The Lon protease is a AAA+ protein found in prokaryotes, archaea, and eukaryotic organelles. Lon is involved in cellular protein homeostasis by degrading damaged or misfolded abnormal proteins, which prevents these unwanted protein species from forming toxic aggregates. Lon is known to form a homohexamer; each protomer is composed of multiple domains, including an N-terminal substrate-binding globular domain (NGD), a long-helix domain (LH), a three-helix bundle (3H), a AAA+ ATPase module, and a protease domain. We show here, using cryo-electron microscopy (cryo-EM), that the activation process of the Lon AAA+ protease may involve a pentameric assembly and a substrate-dependent incorporation of the sixth protomer to form the substrate-pore-loop contacts seen in the translocating state.

To create monomeric mutants, we designed ΔN-E613K and ΔN-L708R mutations, each of which would introduce a positive charge to the hydrophobic interface. If the ΔN-E613K and ΔN-L708R proteins are monomeric, they are expected to bind next to Ob5 and Ob1, respectively, of the open-spiral pentamer to form inactive hexamers. We solved the cryo-EM structure of ΔN-E613K in complex with MtaLon-Y224S. The structure forms a distinct spiral hexameric complex, in which ΔN-E613K binds next to Ob5 of the pentameric assembly, which is consistent with the predicted binding mode. This heteromeric hexamer distinguishes from the native spiral hexameric form, where the protomer Ac6* binds next to Ob1. The heterocomplex also adopts an auto-inhibited spiral structure; however, unlike the native spiral hexamer, the 3H subdomain of Ob1 rather than Ac6* occupies the axial cavity of the spiral complex. In these structures, the protease domain of ΔN-E613K and the AAA+ domain of Ac6* engage heterotypic interactions with the AAA+ domain of Ob1 and the protease domain of Ob5, respectively. Altogether, these results demonstrate the binding of a monomeric mutant to the pentameric Lon, which results in a 5+1 heteromeric complex. The heteromeric complexes containing the incorporated monomeric ΔN-E613K or ΔN-L708R are expected to be non-functional as they are unable to form a closed-ring structure due to the mutated residues at the binding interface.

>[5x]MRLELPVIPLRNTVILPHTTTPVDVGRAKSKRAVEEAMGADRLIFLVAQRDPEVDDPAPDDLYTWGVQAVVKQAMRLPDGTLQVMVEARARAQVTDYIPGPYLRARGEVFSEIFPIDEAVVRVLVEELKEAFEKYVANHKSLRLDRYQLEAVKGTSDPAMLADTIAYHATWTVAEKQEILELTDLEARLKKVLGLLSRDLERFELDKRVAQRVKEQMDTNQRESYLREQMKAIQKELGGEDGLSDLEALRKKIEEVGMPEAVKTKALKELDRLERMQQGSPEATVARTYLDWLTEVPWSKADPEVLDINHTRQVLDEDHYGLKDVKERILEYLAVRQLTQGLDVRNKAPILVLVGPPGVGKTSLGRSIARSMNRKFHRISLGGVRDEAEIRGHRRTYIGAMPGKLIHAMKQVGVINPVILLDEIDKMSSDWRGDPASAMLEVLDPEQNNTFTDHYLDVPYDLSKVFFITTANTLQTIPRPLLDRMEVIEIPGYTNMEKQAIARQYLWPKQVRESGMEGRIEVTDAAILRVISEYTREAGVRGLERELGKIARKGAKFWLEGAWEGLRTIDASDIPTYLGIPRYRPDKAETEPQVGTAQGLAWTPVGGTLLTIEVAAVPGSGKLSLTGQLGEVMKESAQAALTYLRAHTQDYGLPEDFYNKVDLHVHVPDGATPKDGPSAGITMATAIASALSRRPARMDIAMTGEVSLRGKVMPIGGVKEKLLAAHQAGIHKIVLPKDNEAQLEELPKEVLEGLEIKLVEDVGEVLEYLLLPEPTMPPVVQPSDNRQQPGAGAHHHHHH;> HHHHHHSSGENLYFQGHMGLSDLEALRKKIEEVGMPEAVKTKALKELDRLERMQQGSPEATVARTYLDWLTEVPWSKADPEVLDINHTRQVLDEDHYGLKDVKERILEYLAVRQLTQGLDVRNKAPILVLVGPPGVGKTSLGRSIARSMNRKFHRISLGGVRDEAEIRGHRRTYIGAMPGKLIHAMKQVGVINPVILLDEIDKMSSDWRGDPASAMLEVLDPEQNNTFTDHYLDVPYDLSKVFFITTANTLQTIPRPLLDRMEVIEIPGYTNMEKQAIARQYLWPKQVRESGMEGRIEVTDAAILRVISEYTREAGVRGLERELGKIARKGAKFWLEGAWEGLRTIDASDIPTYLGIPRYRPDKAETEPQVGTAQGLAWTPVGGTLLTIKVAAVPGSGKLSLTGQLGEVMKESAQAALTYLRAHTQDYGLPEDFYNKVDLHVHVPDGATPKDGPSAGITMATAIASALSRRPARMDIAMTGEVSLRGKVMPIGGVKEKLLAAHQAGIHKIVLPKDNEAQLEELPKEVLEGLEIKLVEDVGEVLEYLLLPEPTMPPVVQPSDNRQQPGAGA(2~{S})-2-oxidanyl-2-(3-phenoxyphenyl)ethanoic acid | C14 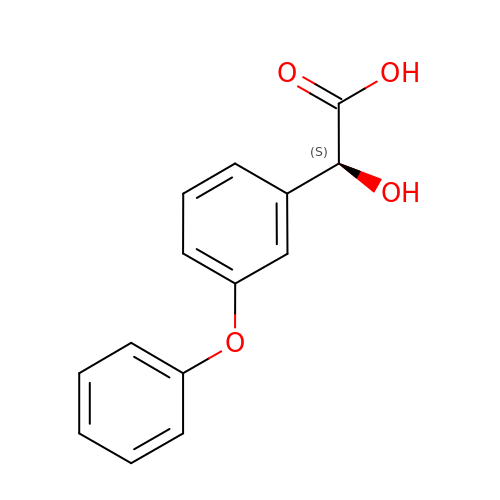H12 O4 | FPUCYPXKIFVDSD-ZDUSSCGKSA-N>MFDPAEKYKMDHRRRGIALIFNHERFFWHLTLPERRGTCADRDNLTRRFSDLGFEVKCFNDLKAEELLLKIHEVSTVSHADADCFVCVFLSHGEGNHIYAYDAKIEIQTLTGLFKGDKCHSLVGKPKIFIIQACRGNQHDVPVIPLDVVD[4x];>MAASVYTLPAGADFLMCYSVAEGYYSHRETVNGSWYIQDLCEMLGKYGSSLEFTELLTLVNRKVSQRRVDFCKDPSAIGKKQVPCFASMLTKKLHFFPKSNLEHHHHHH[4x]

Caspases are cysteine-dependent aspartyl-specific proteases involved in a range of cellular and disease processes, ranging from apoptosis to inflammation and neurodegeneration. Caspase family members are broadly classified as inflammatory (C1, C4, and C5) or apoptotic caspases. While often classified as an executioner caspase, the function of caspase-6 (C6) in physiology and disease has remained enigmatic, and it has been suggested that C6 may act upstream of the other executioner caspases. C6 possesses a non-catalytic cysteine (C264) not present in other family members and is situated on a loop in the small subunit at the distal end of the active site. The catalytic cysteine (C163) is found on the large subunit, while two additional cysteine residues appear to be buried and thus inaccessible for disulfide formation.

One successful foray in this vein produced analogue 2a (R = p-OCF3), in which the nipecotic acid core was reoriented, with the piperidine nitrogen displaying a vinylsulfonamide. Analogue 2a, having the 3R configuration, exhibited markedly superior C264 engagement compared to its 3S enantiomer 2b, with a mass spectrometry-based dose–response-50 (DR50) value of 0.08 μM and a C6 inhibition IC50 value of 0.180 μM, indicating that inhibition by 2a involved both molecular recognition and reaction with C264. The crystal structure of 2a bound to C6 confirmed the covalent modification of residue C264, whose α-carbon atom moved ∼2.4 Å toward the substrate-binding groove, compared to the structure of C6 bound to a VEID peptide substrate analogue. Informed by this structure, we explored new piperidine substitutions, seeking to engage additional pockets in the active site. A complex X-ray crystal structure of 3a showed similarities and differences as compared to the binding of 2a. Both analogues engaged C264 in a covalent bond as expected, while the trifluoromethoxyaryl side chain of both analogues was buried in the S1 pocket, where the aspartic acid residue of the C6 substrate is usually bound. However, the location and orientation of the piperidine ring and sulfonamide function were quite different in the two analogues. Lamin A cleavage was inhibited by 2a with an IC50 value of 14.2 ± 2.4 μM and by 3a with an IC50 value of 170 ± 4 nM. Importantly, 2a and 3a inhibited lamin A cleavage in a manner that tracked well with their biochemical potencies, with 2a roughly 50-fold less potent than 3a.[(2~{R},3~{S},4~{S},5~{R})-3,4-bis(oxidanyl)-5-[3-(4-pyridin-3-yl-1,2,3-triazol-1-yl)propyl]oxan-2-yl]methyl ~{N}-[(2~{S})-2-azanyl-4-methyl-pentanoyl]sulfamate | C22 H34 N6 O7 S | 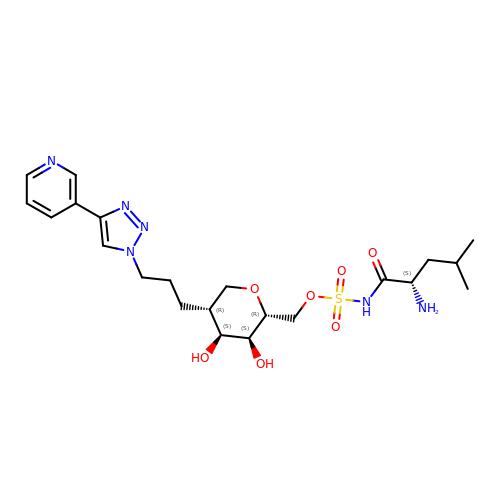ADQFJUZJIVRSDT-LXDWIVHCSA-N> VDICTAKPRDIPMNPMCIYRSPEKKATEDEGSEQKIPEATNRRVWELSKANSRFATTFYQHLADSKNDNDNIFLSPLSISTAFAMTKLGACNDTLQQLMEVFKFDTISEKTSDQIHFFFAKLNCRLYRKAAKSSKLVSANRLFGDKSLTFNETYQDISELVYGAKLQPLDFKENAEQSRAAINKWVSNKTEGRITDVIPSEAINELTVLVLVNTILFKGLWKSKFSPENTRKELFYKADGESCSASMMYQEGKFRYRRVAEGTQVLELPFKGDDITMVLILPKPEKSLAKVEKELTPEVLQEWLDELEEMMLVVHMPRFRIEDGFSLKEQLQDMGLVDLFSPEKSKLPGIVAEGRDDLYVSDAFHKAFLEVNEEGSEAAASTAVVIAGRSLNPNRVTFKANRPFLVFIREVPLNTIIFMGRVANPCV;> VDICTAKPRDIPMNPMCIYRSPEKKATEDEGSEQKIPEATNRRVWELSKANSRFATTFYQHLADSKNDNDNIFLSPLSISTAFAMTKLGACNDTLQQLMEVFKFDTISEKTSDQIHFFFAKLNCRLYRKANKSSKLVSANRLFGDKSLT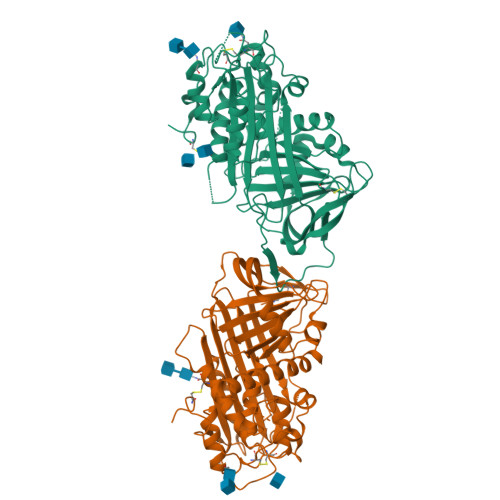FNETYQDISELVYGAKLQPLDFKENAEQSRAAINKWVSNKTEGRITDVIPSEAINELTVLVLVNTIYFKGLWKSKFSPENTRKELFYKADGESCSASMMYQEGKFRYRRVAEGTQVLELPFKGDDITMVLILPKPEKSLAKVEKELTPEVLQEWLDELEEMMLVVHMPRFRIEDGFSLKEQLQDMGLVDLFSPEKSKLPGIVAEGRDDLYVSDAFHKAFLEVNEEGSEAAASTAVVIAGRSLNPNRVTFKANRPFLVFIREVPLNTIIFMGRVANPCV>GSIQQATTGVSQETSENPGDKTIVPATLPQLTPTLVSLLEVIEPEVLYAGYDSSVPDSTWRIMTTLNMLGGRQVIAAVKWAKAIPGFRNLHLDDQMTLLQYSWMSLMAFALGWRSYRQSSANLLCFAPDLIINEQRMTLPDMYDQCKHMLYVSSELHRLQVSYEEYLCMKTLLLLSSVPKDGLKSQELFDEIRMTYIKELGKAIVKREGNSSQNWQRFYQLTKLLDSMHEVVENLLNYCFQTFLDKTMSIEFPEMLAE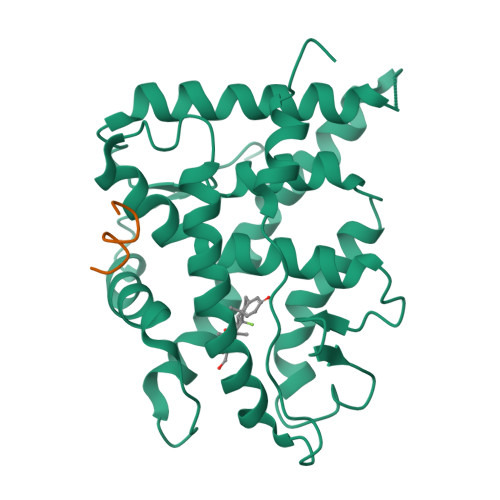IITNQIPKYSNGNIKKLLFHQK[4x];>KENALLRYLLDK[4x]>[3x]MGHMPSLHNIPVPETNYLGNTPTMPFSSLPPTDESIKYTIYNSTGIQIGAYNYME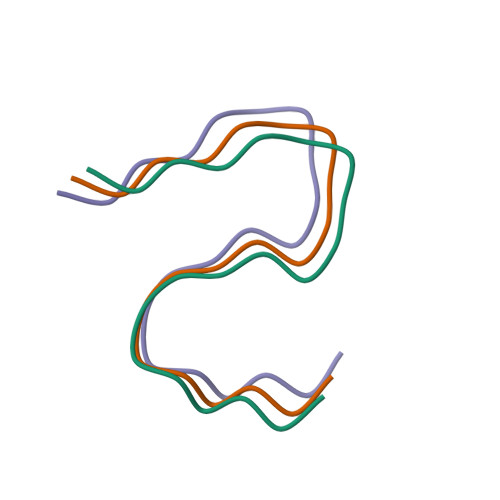IGGTSSSLLDSTNTNFKEEPAAKYQAIFDNTTSLTLEHHHHHH>[3x]GTHHHHHHHHGSQNETEPIVLEGKCLVVCDSNPTSDPTGTALGISVRSGSAKVAFSAIRSTNHEPSEMSNRTMIIYFDQVLVNIGNNFDSERST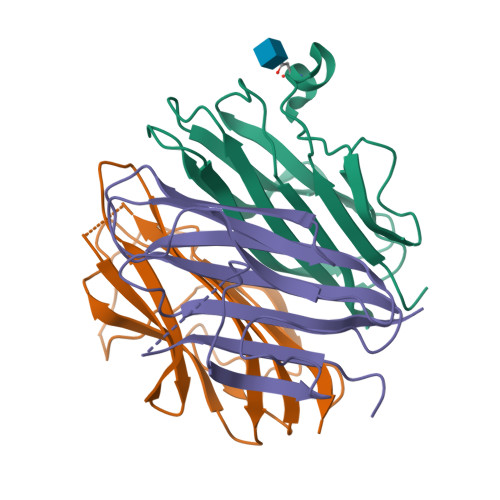FIAPRKGIYSFNFHVVKVYNRQTIQVSLMLNGWPVISAFAGDQDVTREAASNGVLIQMEKGDRAYLKLERGNLMGGWKYSTFSGFLVFPL>[2x]MKMYEVKEFSSGKRKLEDYKSIIGEEEVSKIQEKAEKLKGRSFVHVNSTSFGGGVAEILHSLVPLLRSIGIEARWFVIEGPTEFFNVTKTFHNALQGNESLKLTEEMKELYLNVNRENSKFIDLSSFDYVLVHDPQPAALIEFYEKKSPWLWRCHIDLSSPNREFWEFLR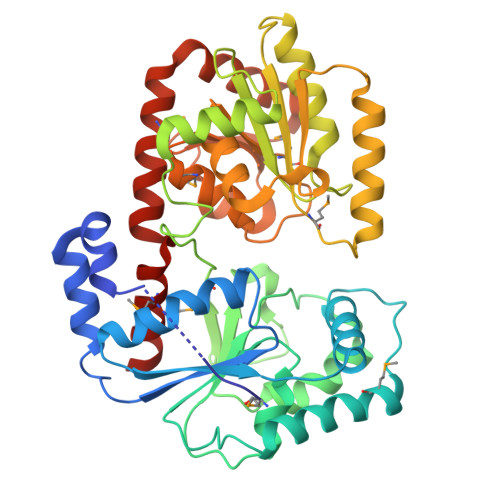RFVEKYDRYIFHLPEYVQPELDRNKAVIMPPSIDPLSEKNVELKQTEILRILERFDVDPEKPIITQVSRFDPWKGIFDVIEIYRKVKEKIPGVQLLLVGVMAHDDPEGWIYFEKTLRKIGEDYDVKVLTNLIGVHAREVNAFQRASDVILQMSIREGFGLTVTEAMWKGKPVIGRAVGGIKFQIVDGETGFLVRDANEAVEVVLYLLKHPEVSKEMGAKAKERVRKNFIITKHMERYLDILNSLGG> MENRWQVM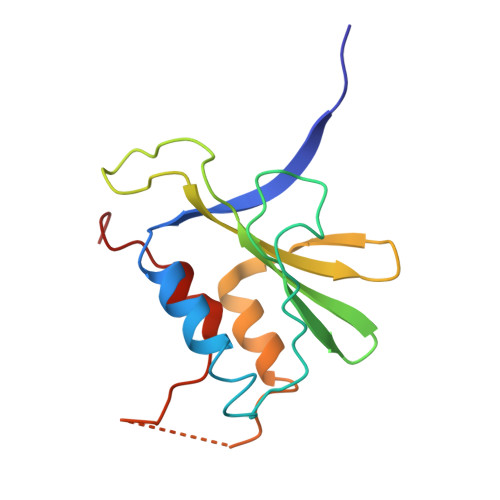IVWQVDRMRINTWKRLVKHHMYISRKAKDWFYRHHYESTNPKISSEVHIPLGDAKLVITTYWGLHTGERDWHLGQGVSIEWRKKRYSTQVDPDLADQLIHLHYFDEASEGSQIKPPLPSVRKLTEDRWNK N-[(3-fluorophenyl)methyl]-N-methylsulfuric diamide | C8 H11 F N2 O2 S | 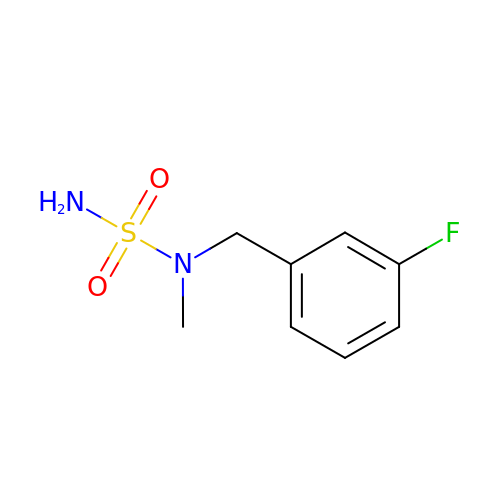MTNUKOMLMCLFRR-UHFFFAOYSA-N1,2-Dioctanoyl-SN-Glycero-3-Phosphoethanolamine 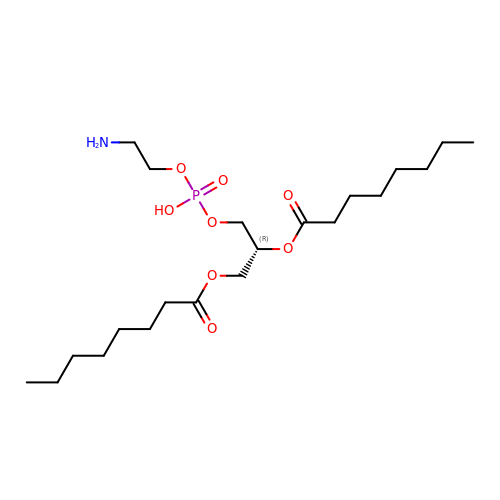| C21 H42 N O8 P | UNACBKDVIYEXSL-LJQANCHMSA-N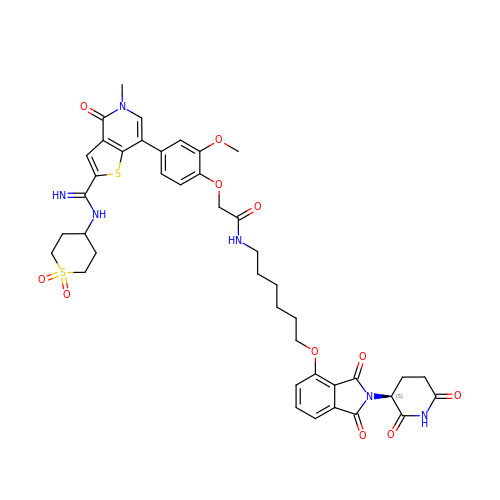N-[6-({2-[(3S)-2,6-dioxopiperidin-3-yl]-1,3-dioxo-2,3-dihydro-1H-isoindol-4-yl}oxy)hexyl]-2-(4-{2-[N-(1,1-dioxo-1lambda~6~-thian-4-yl)carbamimidoyl]-5-methyl-4-oxo-4,5-dihydrothieno[3,2-c]pyridin-7-yl}-2-methoxyphenoxy)acetamide | C42 H46 N6 O11 S2 | KUQBYZITZXQWFL-LJAQVGFWSA-N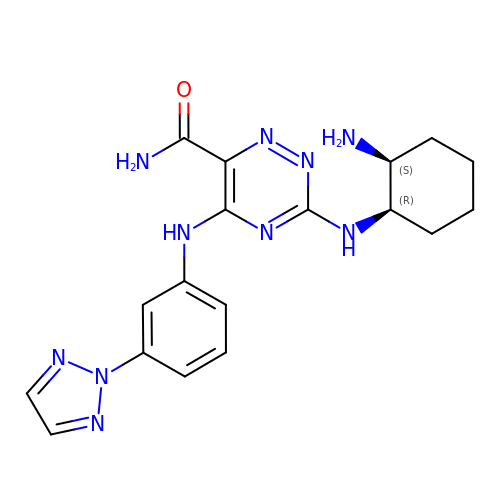3-{[(1R,2S)-2-aminocyclohexyl]amino}-5-{[3-(2H-1,2,3-triazol-2-yl)phenyl]amino}-1,2,4-triazine-6-carboxamide | C18 H22 N10 O | QYUNZLTYDOGJCE-UONOGXRCSA-N Low-density lipoprotein receptor-related protein 6 (LRP6) is a coreceptor of the β-catenin-dependent Wnt signaling pathway. As a member of the LDL receptor family, LRP6 is a single-pass transmembrane protein with a large extracellular domain (ECD) consisting of four repeating units (E1, E2, E3, and E4), each of which has a YWTD β-propeller domain flanked by an epidermal growth factor-like domain. The LRP6 ectodomain binds Wnt proteins, as well as Wnt inhibitors such as sclerostin (SOST), which negatively regulates Wnt signaling in osteocytes. SOST inhibits new bone formation and growth by binding to LRP5/6, thereby inhibiting canonical Wnt signaling in osteoblasts.

The crystal structure of a complex between LRP6 E1E2 and SOSTtr177 (a C-terminal 37-amino acid truncation mutant of SOST) suggested that the C-terminal region of SOST might contribute to LRP6 binding. The mFo-DFc difference electron density map calculated after rigid body fitting of the MR solution revealed clear density for SOST NXI motif at the top surface of LRP6 E1. In our structure, R121 made close contacts with the E73 side chain and the backbone carbonyls of V70 and L95 in LRP6 E1. The shortened C-tail of our SOSTtr177 construct (169-RLTRFHNQS-177) facilitated model building, as we observed a clear side-chain density for H174 at the center of LRP6 E2, where H174 stably interacts with polar residues of LRP6 E2. H174 of SOST made close contacts with R449, W465, W491, N493, and H534 of LRP6. Unexpectedly, in contrast to LRP6 E1, LRP6 E2 showed conformational changes upon SOST binding in that residues at the center of the LRP6 E2 propeller were rearranged to accommodate the insertion of SOST H174. The ligand-binding pocket of the SOST C-tail-bound LRP6 E2 (consisting of W491, N493, R449, and H534) appears remarkably similar to that of the SOST loop 2-bound LRP6 E1. A possibility that a second SOST molecule bound LRP6 E2 was excluded by the fact that 1:1 heterodimer formation was observed for the LRP6 E1E2–SOSTtr177 complex using multi-angle light scattering (MALS) analysis. However, the current structure clearly indicates that SOST interacts with both LRP6 E1 and E2 through loop 2 and C-tail, respectively. First, the SOST loop 2–LRP6 E1 interaction is more extensive than the SOST C-terminal tail–LRP6 E2 interaction (~540 Å2 versus ~400 Å2, respectively).

>ADPLLLYANRRDLRLVDATNGKENATIVVGGLEDAAAVDFVFSHGLIYWSDVSEEAIKRTEFNKTESVQNVVVSGLLSPDGLACDWLGEKLYWTDSETNRIEVSNLDGSLRKVLFWQELDQPRAIALDPSSGFMYWTDWGEVPKIERAGMDGSSRFIIINSEIYWPNGLTLDYEEQKLYWADAKLNFIHKSNLDGTNRQAVVKGSLPHPFALTLFEDILYWTDWSTHSILACNKYTGEGLREIHSDIFSPMDIHAFSQQRQPNATNPCGIDNGGCSHLCLMSPVKPFYQCACPTGVKLLENGKTCKDGATELLLLARRTDLRRISLDTPDFTDIVLQLEDIRHAIAIDYDPVEGYIYWTDDEVRAIRRSFIDGSGSQFVVTAQIAHPDGIAVDWVARNLYWTDTGTDRIEVTRLNGTMRKILISEDLEEPRAIVLDPMVGYMYWTDWGEIPKIERAALDGSDRVVLVNTSLGWPNGLALDYDEGKIYWGDAKTDKIEVMNTDGTGRRVLVEDKIPHIFGFTLLGDYVYWTDWQRRSIERVHKRSAEREVIIDQLPDLMGLKATNVHRVIGSNPCAEENGGCSHLCLYRPQGLRCACPIGFELISDMKTCIVPHHHHHHHHHH[2x];>[2x]GPSRQGWQAFKNDATEIIPELGEYPEPPPELENNKTMNRAENGGRPPHHPFETKDVSEYSCRELHFTRYVTDGPCRSAKPVTELVCSGQCGPARLLPNAIGRGKWWRPSGPDFRCIPDRYRAQRVQLLCPGGEAPRARKVRLVASCKCKRLTRFHNQS> ARLNRESVIDAALELLNETGIDGLTTRKLAQKLGIEQPTLYWHVKNKRALLDALAVEILARHHDYSLPAAGESWQSFLRNNAMSFRRALLRYRDGAKVHLGTRPDEKQYDTVETQLRFMTENGFSLRDGLYAISAVSHFTLGAVL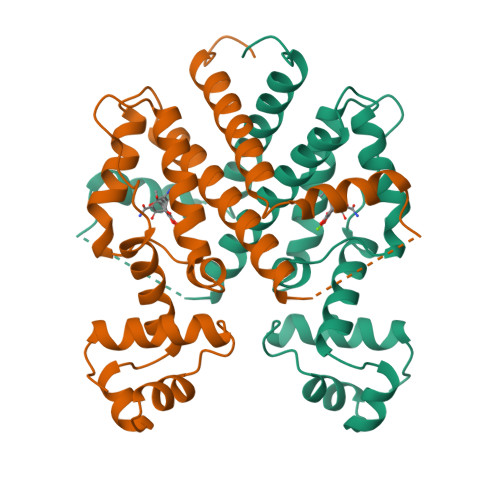EQQEHTAALTDRPAAPDENLPPLLREALQIMDSDDGEQAFLHGLESLIRGFEVQLTALLQIVGGDKLIIPFC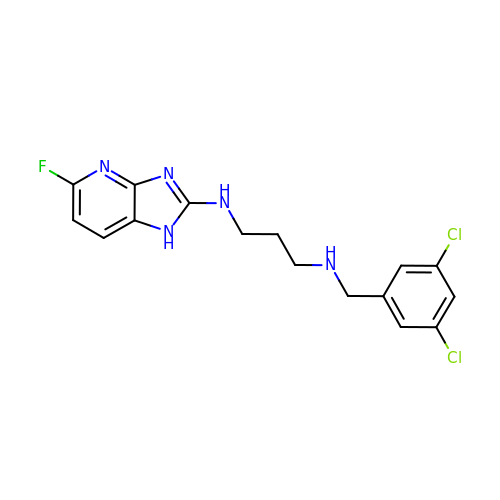N-(3,5-dichlorobenzyl)-N'-(5-fluoro-1H-imidazo[4,5-b]pyridin-2-yl)propane-1,3-diamine | C16 H16 Cl2 F N5 | PLEWLGWDDKXXIA-UHFFFAOYSA-N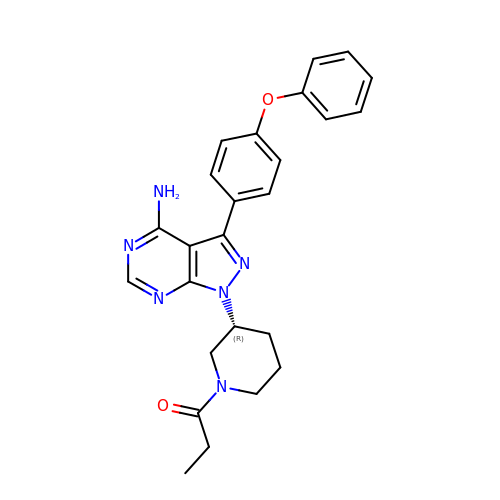1-[(3~{R})-3-[4-azanyl-3-(4-phenoxyphenyl)pyrazolo[3,4-d]pyrimidin-1-yl]piperidin-1-yl]propan-1-one | C25 H26 N6 O2 | ROGRQCNRPWIQJN-GOSISDBHSA-N FLUORESCIN | 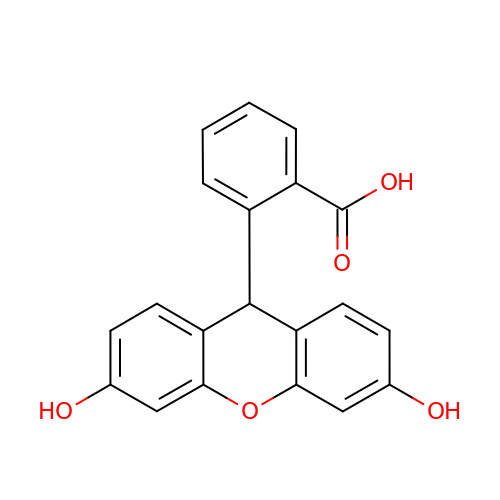C20 H14 O5 | MURGITYSBWUQTI-UHFFFAOYSA-N>[6x]MRIERVDDTTVKLFITYSDIEARGFSREDLWTNRKRGEEFFWSMMDEINEEEDFVVEGPLWIQVHAFEKGVEVTISKSKNEDMMNMSDDDATDQFDEQVQELLAQTLEGEDQLEELFEQRTKEKEAQGSKRQKSSARKNTRTIIVKFNDLEDVINYAYHSNPITTEFEDLLYMVDGTYYYAVYFDSHVDQEVINDSYSQLLEFAYPTDRTEVYLNDYAKIIMSHNVTAQVRRYFPETTE;>[12x]MLFGRLTERAQRVLAHAQEEAIRLNHSNIGTEHLLLGLMKEPEGIAAKVLESFNITEDKVIEEVEKLIGHGQDHVGTLHYTPRAKKVIELSMDEARKLHHNFVGTEHILLGLIRENEGVAARVFANLDLNITKARAQVVKALGNPEMSNKNAQASKSNNTPTLDSLARDLTVIAKDGTLDPV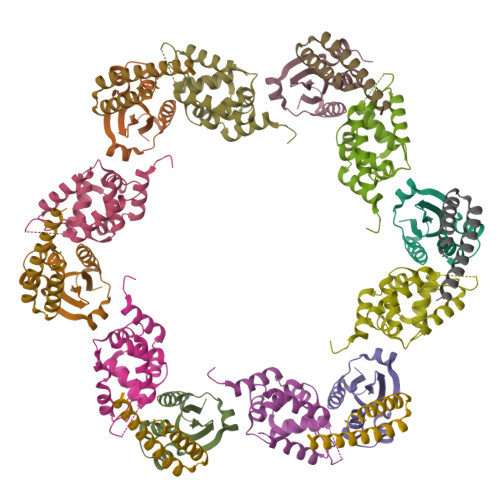IGRDKEITRVIEVLSRRTKNNPVLIGEPGVGKTAIAEGLAQAIVNNEVPETLKDKRVMSLDMGTVVAGTKYRGEFEERLKKVMEEIQQAGNVILFIDELHTLVGAGGAEGAIDASNILKPALARGELQCIGATTLDEYRKNIEKDAALERRFQPVQVDEPSVVDTVAILKGLRDRYEAHHRINISDEAIEAAVKLSNRYVSDRFLPDKAIDLIDEASSKVRLKSHTTPNNLKEIEQEIEKVKNEKDAAVHAQEFENAANLRDKQTKLEKQYEEAKNEWKNAQNGMSTSLSEEDIAEVIAGWTGIPLTKINETESEKLLSLEDTLHERVIGQKDAVNSISKAVRRARAGLKDPKRPIGSFIFLGPTGVGKTELARALAESMFGDDDAMIRVDMSEFMEKHAVSRLVGAPPGYVGHDDGGQLTEKVRRKPYSVILFDEIEKAHPDVFNILLQVLDDGHLTDTKGRTVDFRNTIIIMTSNVGAQELQDQRFAGFGGSSDGQDYETIRKTMLKELKNSFRPEFLNRVDDIIVFHKLTKEELKEIVTMMVNKLTNRLSEQNINIIVTDKAKDKIAEEGYDPEYGARPLIRAIQKTIEDNLSELILDGNQIEGKKVTVDHDGKEFKYDIAEQTSETKTPSQA> HHHHHHHHGSGSVPAGAKCRLVETLPENMDFRSDHLTTFECFNEIITLAKKYIYIASFCCNPLSTTRGALIFDKLKEASEKGIKIIVLLDERGKRNLGELQSHCPDINFITVNIDKKNNVGLLLGCFWVSDDERCYVGNASFTGGSIHTIKTLGVYSDYPPLATDLRRRFDTFKAFNSAKNSAANLASAAAALPVSTAYHIKNPIGGVFFTDSPEHLLGYSRDLDTDVVIDKLKSAKTSIDIEHLAIVPTTRVDGNSYYWPDIYNSIIEAAINRGVKIRLLVGNWDKNDVYSMATARSLDELCVQNDLSVKVFTIQNNTKLLIVDDEYVHITSANFDGTHYQNHGFVSFNSIDKQLVSEAKKIFERDWVSSHSKSLKI

F13 is a phospholipase anchored to membranes via two palmitoylated cysteines located in a hydrophobic membrane-interacting region (MIR). Tecovirimat is an inhibitor of mature virus wrapping widely used to treat mpox patients infected with clade IIb strains. Tecovirimat binding to F13 blocks viral wrapping, but the structural mechanism is poorly understood. We showed that F13 forms a homodimer on membranes, and tecovirimat inserts into a cavity formed between the two protomers.

Next, we aimed to elucidate the structural basis of the partial resistance of the A295E mutant. We obtained cubic crystals of sF13A295E and soaked them in tecovirimat. In the absence of tecovirimat, sF13A295E formed a homodimer that resembled that of sF13WT, but with the ends of the α10 helix being more open, so that Y285 was hydrogen-bonded with Q299 instead of with N300, as in the wild-type protein. In the presence of tecovirimat, sF13A295E recovered the native conformation, in which Y285 was hydrogen-bonded to N300. Overall, we concluded that escape mutants isolated from tecovirimat-treated patients alter the dimerization interface of sF13, making tecovirimat-induced dimerization less efficient. In line with the AUC experiments, tecovirimat induced a strong increase in the PLA signal in cells expressing Flag–F13WT, a slight increase in cells expressing Flag–F13A295E and none in cells expressing Flag–F134MUT.>[60x]GSGVGISTGGWVGGSHFADKYVITKNTRQFITSIQNGHLYKTEIINPSNGNGKSQRCVTTPWTYFNFNQYSCHFSPQDWQRLTNEYKRFRPK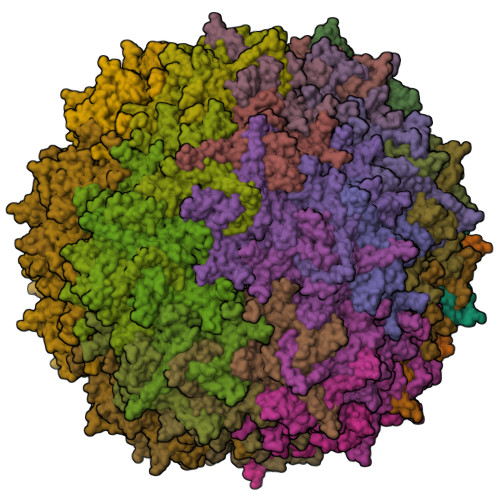AMLVKIYNLQIKQILSNGADTTYNNDLTAGVHIFCDGEHAYPNASHPWDEDVMPDLPYKTWKLFQYGYIPILNELADLDGTTAGGTATEKAILYQMPFFMLENSDHEVLRTGESSEFTFNFDCEWVNNERAYIPPGLMFNPKVPTRRVQYIRQNGQTTASTSRIEPYSKPTSWMTGPGFLGGQRVGPATSDTAPYMVCTKPDGVYINTGAAGYGSGFDPPSGSLAPTDLEYKLQWYQTPEDTGNNGNIIANPSLSMLRDQLLYRGNQTTYNLNADVWMFPNQIWDRYPITREHPIWCKKPRADKNTIIDPFDGSIAMDHPPGTIFIKMAKIPVPSSTNADSYLNIYCTGQVSCEIVWEVERYVTKNWRPERRHTALGMSIGGTENVSPTYHVDSAGTYIQPTTFDQCMPVKTNINKVL>QPTAPKDFSSGFWDFNDGTTQGFGVNPDSPITAINVENANNALKISNLNSKGSNDLSEGNFWANVRISADIWGQSINIYGDTKLTMDVIAPTPVNVSIAAIPQSSTHGWGNPTRAIRVWTNNFVAQTDGTYKATLTI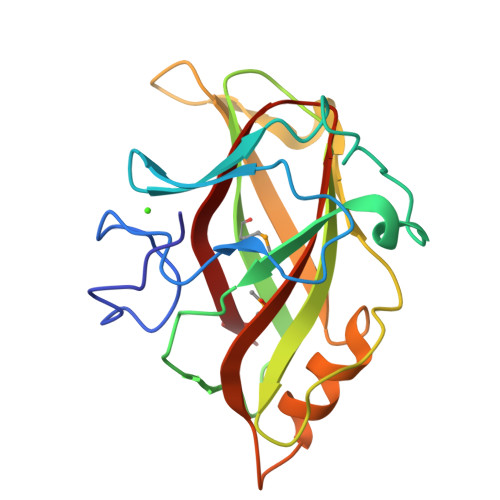STNDSPNFNTIATDAADSVVTNMILFVGSNSDNISLDNIKFTK[2x]>GGGGLEEEFRKLTNVRIMKENMRTGNLPANMKKARVIQIIPYDFNRVILSMKRGQEYTDYINASFIDGYRQKDYFIATQGPLAHTVEDFWRMIWEWKSHTIVMLTEVQEREQDKCYQYWPTEGSVTHGEITIEIKNDTLSEAISIRDFLVTLNQPQARQEEQVRVVRQFHFHGWPEIGIPAEGKGMIDLIAAVQKQQQQ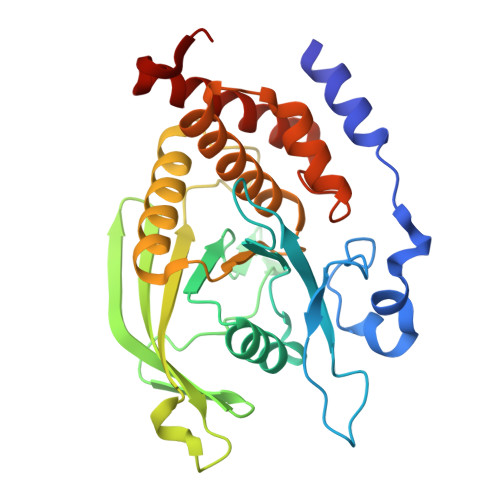TGNHPITVHCSAGAGRTGTFIALSNILERVKAEGLLDVFQAVKSLRLQRPHMVQTLEQYEFCYKVVQDFIDIFSDYANFK[2x]> HHHHHHPPCETHETGTTNTATTATGGGTHADSLNNLANIKREQGNIEEAVRLYRKALEVFPEFAAAHSNLASVLQQQGKLQEALMHYKEAIRISPTFADAYSNMGNTLKEMQDVQGALQCYTRAIQINPAFADAHSNLASIHKDSGNIPEAIASYRTALKLKPDFPDAYCNLAHCLQIVCDWTDYDERMKKLVSIVADQLEKNRLPSVHPHHSMLYPLSHGFRKAIAERHGNLCLDKINVLHKPPYEHPKDLKLSDGRLRVGYVSSDFGNHPTSHLMQSIPGMHNPDKFEVFCYALSPDDGTNFRVKVMAEANHFIDLSQIPCNGKAADRIHQDGIHILVNMNGYTKGARNELFALRPAPIQAMWLGYPGTSGALFMDYIITDQETSPAEVAEQYSEKLAYMPHTFFIGDHANMFPHLKKKAVIDFKSNGHIYDNRIVLNGIDLKAFLDSLPDVKIVKMKCPDGGDNADSSNTALNMPVIPMNTIAEAVIEMINRGQIQITINGFSISNGLATTQINNKAATGEEVPRTIIVTTRSQYGLPEDAIVYCNFNQLYKIDPSTLQMWANILKRVPNS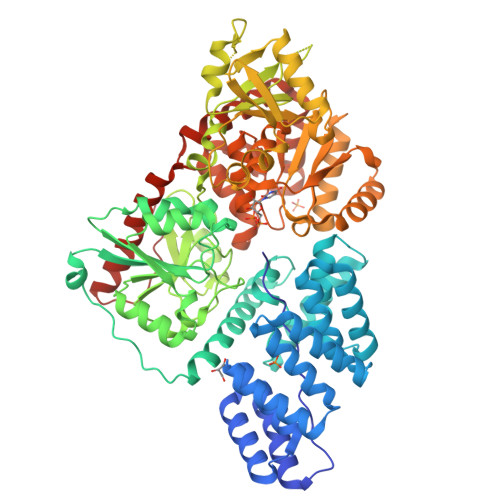VLWLLRFPAVGEPNIQQYAQNMGLPQNRIIFSPVAPKEEHVRRGQLADVCLDTPLCNGHTTGMDVLWAGTPMVTMPGETLASRVAASQLTCLGCLELIAKNRQEYEDIAVKLGTDLEYLKKVRGKVWKQRISSPLFNTKQYTMELERLYLQMWEHYAAGNKPDHMIKPVEVTESA> MDKEIYCGSVPVSYFDPFDLFESLRPEFQQILPLDNIHWKAFDGTVRTVNRLPIELIPEGRGEADKSNDEQPFIRFLIVNCISIDQYRAKVRPLVRQWLPNLESVSSSTGEKMIYKPIILLYANSEVVDSNLFKSVSLMEKFGKDFPHVQTLEVRSVYRSPKERQEFWNQFSQKIKASVLSIFQKRLTHLQHSLANLQKGNNFEEQLLTREKLYELYVVFNILEDASLELQKIKKEILRRNMNMPDGKLQVPFESSSKSDESLGSIIIEGTLDKFQLHKYFFIRRLRLLKLEDQTLTAFVGAFQLIKNFIESISIEYRKSVRLLEFKHYFITSMLSYFEFENVSNPLLCEIKAELLMLKRDNWVQGVMATSGYRLMDKNYPNSDVKYKFDLLKETFVDETVFQENFLTLTKEILSLFNKCEGKRQRIVDILSIEIGLLYYQGKKYEEAVSLFLSCYEYYTQTNWNSIGLKILQVFIDSLSHCPKLDVLQIDGESVSASAVLTNAFLNILKLCKDNDSKEIWWKKFMDLQMKNNIHLMYPLDGLFEVTLNSKVHLARANVSAIEVNLKSYGFPEDISTKTMRLSLKNMGGDVIVFGASDFLLKKGENKLILECRDIMYGEFSLLSFEIIVEGITFVKEFPENQDEFIVVPEIYCKESTKVLVKQAHNLNLGEYALELKSVQSDALESLQVEVEVQKNIGNMKNLPVSFSMDEIQARKRYNTPFENVRLEYYLLDQITAFDLIIKTSFTKKNDQGTFGETKKVRIQCYLQLSVSVEDIFKKDIFFFKFLLNSSVREEPVILYSSELSAPDTRNDYNIRGDYIATTPALITFDGNESFINCYEITANNNFDSKDIFNLKVRYNTLKEQLDCFITDAVLIEGDVEWFILFEKWKTFWELEILKKLKYDYDAFKENRIIRLLKTSIDLNKTKSKIRNLCIEKAVLDKILICLNKVSRGIAVCNTDMDEYVRNLVPKQLTVPVQLPGFEQFFHVQFEQMETSHDALHDTIATIGNSLSYTVIVENLSGQWGQDV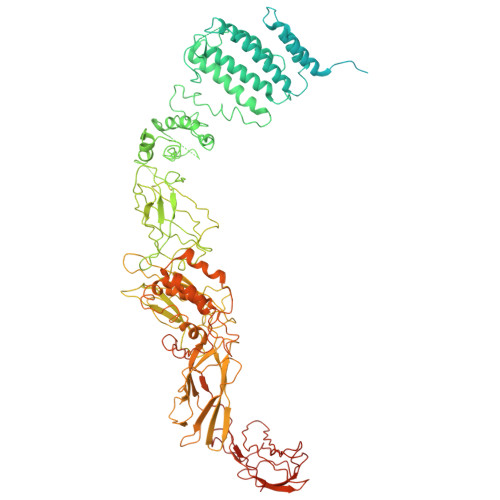IDDGGYIFEILSSNEWLIHGQKRCAIKEKRKEFEVHLIPLKKGYLNFPRVEITNINGKSCRVDHSNAFESILIF>[2x]STAGKVIKCKAAVLWEEKKPFSIEEVEVAPPKA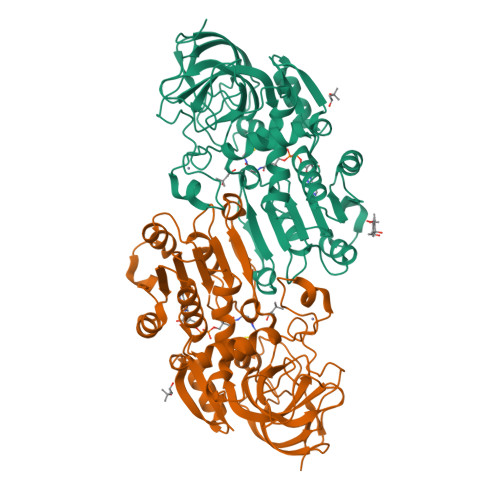HEVRIKMVATGICRSDDHVVSGTLVTPLPVIAGHEAAGIVESIGEGVTTVRPGDKVIPLFTPQCGKCRVCKHPEGNFCLKNDLSMPRGTMQDGTSRFTCRGKPIHHFLGTSTFSQYTVVDEISVAKIDAASPLEKVCLIGCGFSTGYGSAVKVAKVTQGSTCAVFGLGGVGLSVIMGCKAAGAARIIGVDINKDKFAKAKEVGATECVNPQDYKKPIQEVLTEMSNGGVDFSFHVIGRLDTMVTALSCCQEAYGVSVIVGVPPDSQNLSMNPMLLLSGRTWKGAIFGGFKSKDSVPKLVADFMAKKFALDPLITHVLPFEKINEGFDLLRSGESIRTILTF>GAMAIPKIASYQVLPLESFPTNKVDWVIDPKKSVVLVHDLQAYFLNFFDKTLSPVPELLRNVNKVTESARSAGIPVVYTAQPANQDPNERALLTDFWGVGLTQDTEIVPEVSPQPEDIQYTKWRYSAFKKT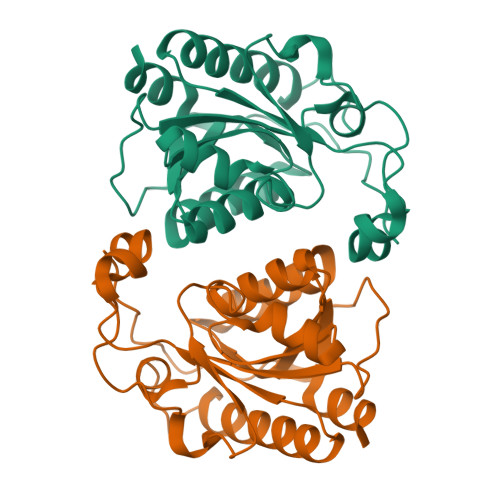PLLEWMKEEQRDQLVIVGVYGHIGILSTALDAFMLDIKPFVIGDAIADFSKEDHMNTLKYVASRSGSVKSVDEFIDSVTTRSFGELS[2x]>[4x]GPMPGKSVVARVAEA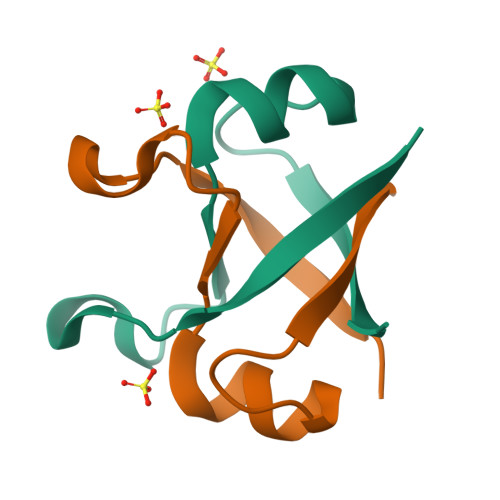YAEDVGKRIVRMDKYERAKLGVSVGDYVEVKKV>MDVNVRGPDGFTPLMIASCSGGGLETGNSEEEEDAPAVISDFIYQGASLHNQTDRTGATALHLAAAYSRSDAAKRLLEASADANIQDNMGRTPLHAAVSADAQGVFQILIRNRATDLDARMHDGTTPLILAARLAV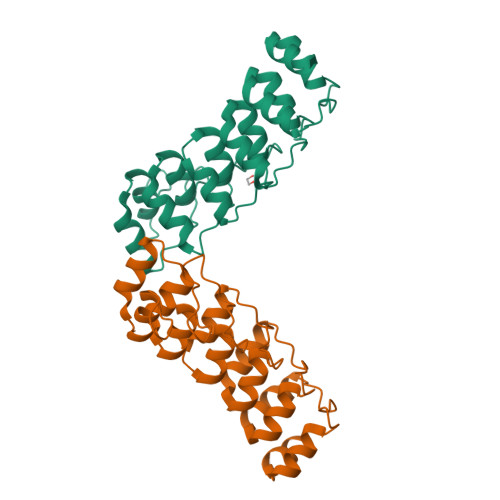EGMLEDLINSHADVNAVDDLGKSALHWAAAVNNVDAAVVLLKNGANKDMQNNREETPLFLAAREGSYETAKVLLDHFANRDITDHMDRLPRDIAQERMHHDIVRLLDLEHHHHHHHH[2x]>[2x]ADWGPCRTASGDPFIFVTSFTKNIQNPTDNVTGQTYPDFYQWALGDKYSGVCECPSPNPTEARPTLYKTESTLAAGHNSTYFKITNNLEVSTRVYIANV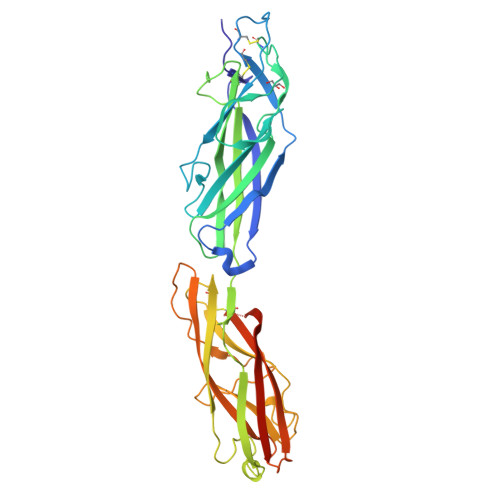GNVQVPFINKSNSQPGRECDQPTFGWTTGSKGQLSLYIAKPFVGEQNIPQTIIVSVFGTKKENVYSSVPISQVLLSGKVTVTQGCELAAGTSLDIDFGEYQAHDFKGRTGQPPQNVQKIQKELTFNCTNISDGVHIYLSLEGTPNAAYPSAISLGNADVGAVIEDGKGNILKPNDSNSLLEMNPGSLYEYVKRKVTTTITAYPVSTTGKLPAAGDYSGVATMHVELDGGGGGGGGGGATTDLGAKGTLKFSLKISQGHHHHHH>[2x]MGHHHHHHGSDPNEAVREFAKEIDVSFVKIEEVIGAGEFGEVYKGRLKLPGKREIYVAIKTLKAGYSEKQRRDF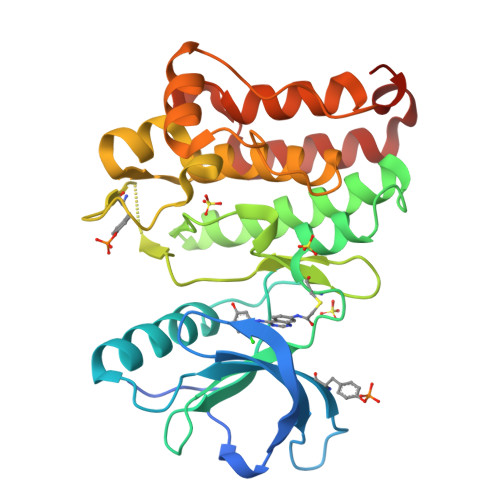LSEASIMGQFDHRNIIRLEGVVTKSRPVMIITEFMENCALDSFLRQNDGQFTVIQLVGMLRGIAAGMKYLSEMNYVHRDLAARNILVNSNLVCKVSDFGLSRYLQDDTSDPTYTSSLGGKIPVRWTAPEAIAYRKFTSASDVWSYGIVMWEVMSFGERPYWDMSNQDVINAIEQDYRLPPPMDCPAALHQLMLDCWQKDRNSRPRFAEIVNTLDKMIRNPASLKTVATITA> MSYVPHVPYVPTPEKVVRRMLEIAKVSQDDIVYDLGCGDGRIIITAAKDFNVKKAVGVEINDERIREALANIEKNGVTGRASIVKGNFFEVDISEATVVTMFLLTNVNEMLKPKLEKELKPGTRVVSHE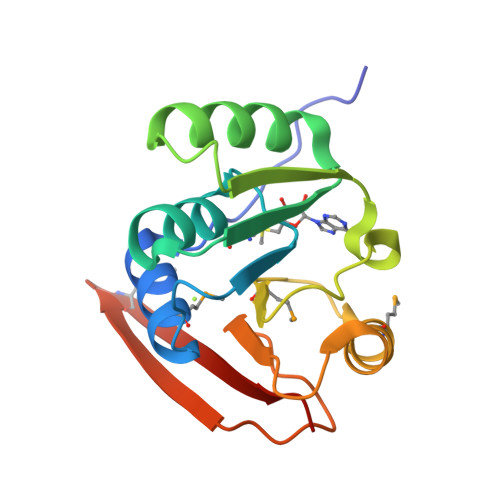FEIRGWNPKEVIKVEDGNMNHTVYLYVIGEHK> DYKDDDDKAEVKKIPTMIEGFDDISHGGLPQGATTLVSGTSGTGKTLFAVQFLYNGITIFNEPGIFVTFEESPQDIIKNALSFGWNLQSLIDQGKLFILDASPDPDGQEVAGDFDLSALIERIQYAIRKYKATRVSIDSVTAVFQQYDAASVVRREIFRLAFRLAQLGVTTIMTTERVDEYGPVARFGVEEFVSDNVVILRNVLEGERRRRTVEILKLRGTTHMKGEYPFTIN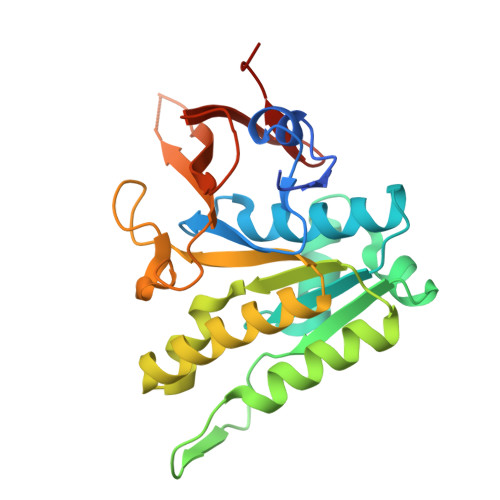NGINIFDYKDDDDK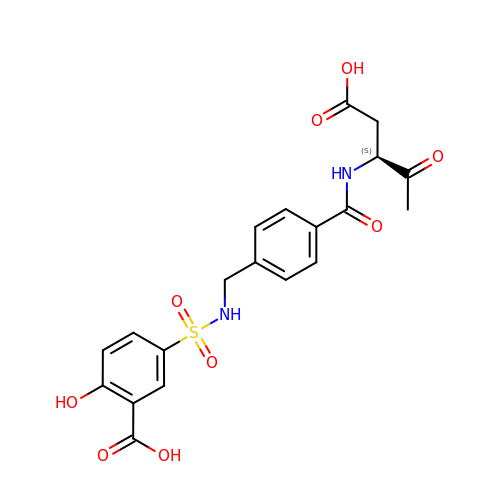5-[4-(1-CARBOXYMETHYL-2-OXO-PROPYLCARBAMOYL)-BENZYLSULFAMOYL]-2-HYDROXY-BENZOIC ACID | C20 H20 N2 O9 S | LBAHOXPDTNUYCX-INIZCTEOSA-N>MQTEHVILLNAQGVPTGTL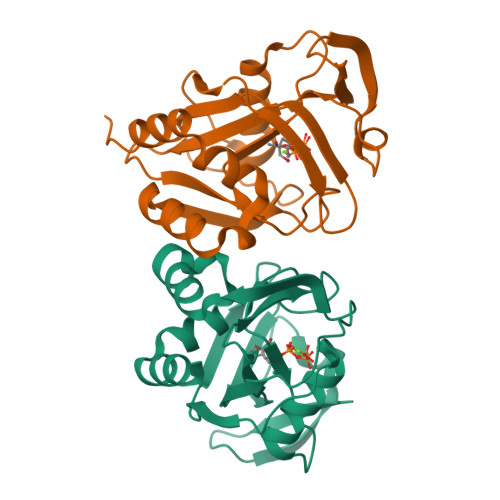EKYAAHTADTRLHLAFSSWLFNAKGQLLVTRRALSKKAWPGVWTNSVAGHPQLGESNEDAVIRRCRYELGVEITPPESIYPDFRYRATDPSGIVENEVCPVFAARTTSALQINDDEVMDYQWCDLADVLHGIDATPWAFSPWMVMQATNREARKRLSAFTQLKL[2x]>[3x]MIQGVIQKIAGPAVIAKGMLGARMYDICKVGEEGLVGEIIRLDGDTAFVQVYEDTSGLKVGEPVVSTGLPLAVELGPGMLNGIYDGIQRPLERIREKTGIYITRGVVVHALDREKK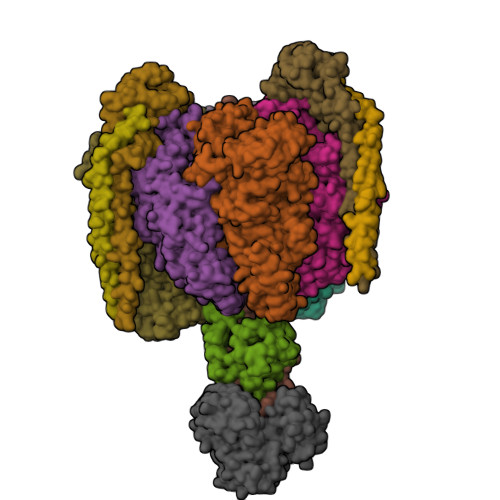WAWTPMVKPGDEVRGGMVLGTVPEFGFTHKILVPPDVRGRVKEVKPAGEYTVEEPVVVLEDGTELKMYHTWPVRRARPVQRKLDPNTPFLTGMRILDVLFPVAMGGTAAIPGPFGSGKTVTQQSLAKWSNADVVVYVGCGERGNEMTDVLVEFPELTDPKTGGPLMHRTVLIANTSNMPVAAREASIYVGVTIAEYFRDQGFSVALMADSTSRWAEALREISSRLEEMPAEEGYPPYLAARLAAFYERAGKVITLGGEEGAVTIVGAVSPPGGDMSEPVTQSTLRIVGAFWRLDASLAFRRHFPAINWNGSYSLFTSALDPWYRENVAEDYPELRDAISELLQREAGLQEIVQLVGPDALQDAERLVIEVGRIIREDFLQQNAYHEVDAYCSMKKAYGIMKMILAFYKEAEAAIKRGVSIDEILQLPVLERIGRARYVSEEEFPAYFEEAMKEIQGAFKALA;>MDLLKKEYTGITYISGPLLFVENAKDLAYGAIVDIKDGTGRVRGGQVIEVSEEYAVIQVFEETTGLDLATTSVSLVEDVARLGVSKEMLGRRFNGIGKPIDGLPPITPEKRLPITGLPLNPVARRKPEQFIQTGISTIDVMNTLVRGQKLPIFSGSGLPANEIAAQIARQATVRPDLSGEGEKEEPFAVVFAAMGITQRELSYFIQEFERTGALSRSVLFLNKADDPTIERILTPRMALTVAEYLAFEHDYHVLVILTDMTNYCEALREIGAAREEIPGRRGYPGYMYTDLATIYERAGVVEGKKGSVTQIPILSMPDDDRTHPIPDLTGYITEGQIQLSRELHRKGIYPPIDPLPSLSRLMNNGVGKGKTREDHKQVSDQLYSAYANGVDIRKLVAIIGEDALTENDRRYLQFADAFERFFINQGQQNRSIEESLQIAWALLSMLPQGELKRISKDHIGKYYGQKLEEIWGAPQALD[3x];> MSQVSPTRMNLLQRRGQLRLAQKGVDLLKKKRDALVAEFFGLVREAMEARKALDQAAKEAYAALLLAQAFDGPEVVAGAALGVPPLEGVEAEVENVWGSKVPRLKATFPDGALLSPVGTPAYTLEASRAFRRYAEALIRVANTETRLKKIGEEIKKTTRRVNALEQVVIPGIRAQIRFIQQVLEQREREDTFRLKRIKGKIEAREAEEEGGRPNPQVEIGAGL;> MAVIADPETAQGFRLAGLEGYGASSAEEAQSLLETLVERGGYALVAVDEALLPDPERAVERLMRGRDLPVLLPIAGLKEAFQGHDVEGYMRELVRKTIGFDIKL;>MTGGLVLNAISRAGGAMGGLGLIKSLAEKEKQLLERLEAAKKEAEERVKRAEAEAKALLEEAEAKAKALEAQYRERERAETEALLARYRERAEAEAKAVREKAMARLDEAVALVLKEVLP[2x];>MSKLEAILSQEVEAEIQALLQEAEAKAEAVKREAEEKAKALLQARERALEAQYRAALRRAESAGELLVATARTQARGEVLEEVRRRVREALEALPQKPEWPEVVRKLALEALEALPGAKALVANPEDLPHLEAMARERGVELQAEPALRLGVRAVGAEGKTQVENSLLARMDRAWDAMSSKVAQALWG[2x];> MADDFAYLNARVRVRRGTLLKESFFQEALDLSFADFLRLLSETVYGGELAGQGLPDVDRAVLRTQAKLVGDLPRLVTGEAREAVRLLLLRNDLHNLQALLRAKATGRPFEEVLLLPGTLREEVWRQAYEAQDPAGMAQVLAVPGHPLARALRAVLRETQDLARVEALLAKRFFEDVAKAAKGLDQPALRDYLALEVDAENLRTAFKLQGSGLAPDAFFLKGGRFVDRVRFARLMEGDYAVLDELSGTPFSGLSGVRDLKALERGLRCVLLKEAKKGVQDPLGVGLVLAYVKEREWEAVRLRLLARRAYFGLPRAQVEEEVVCP>AMADLEQKVLEMEASTYDGVFIWKISDFPRKRQEAVAGRIPAIFSPAFYTSRYGYKMCLRIYLNGDGTGRGTHLSLFFVVMKGPNDALLRWPFNQKVTLMLLDQNNREHVIDAFRPDVTSSSFQRPVNDMNIASGCPLFCPVSKMEAKNSYVRDDAIFIKAIVDLTGL[3x];>[2x]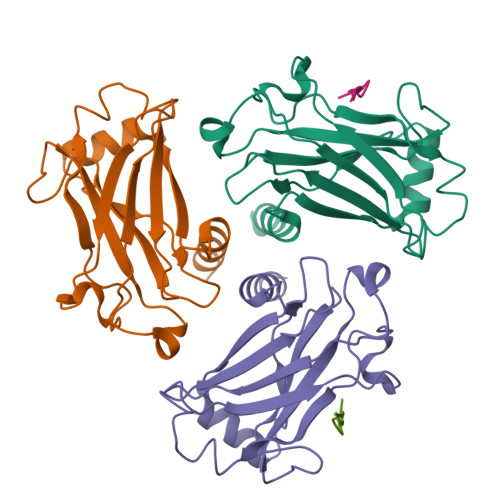XPQQATDD>GSSMASGISVEELLKLAKAAYYSGTTVEEAYKLALKLGISVEELLKLAEAAYYSGTTVEEAYKLALKLGISVEELLKLAKAAYYSGTTVEEAYKLALKLGISVEELLKLAKAAYYSGTTVEEAYKLALKLGISVEELLKLAEAAYYSGTTVEEAYKLALKLGISVEELLKLAKAAYYSGTTVEEAYKLALKLGISVEELLKLAKAAYYSGTTVEEAYKLALKLGISVEELLKLAEAAYYSGTTVEEAYKLALKLGISVEELLKLAKAAYYSGTTVEEAYKLALKLGISVEELLKLA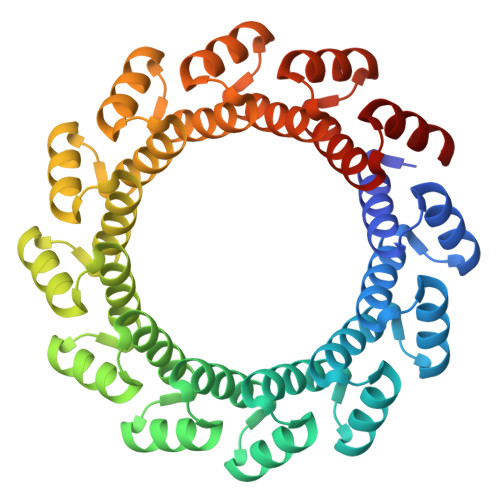KAAYYSGTTVEEAYKLALKLGISVEELLKLAEAAYYSGTTVEEAYKLALKLGISVEELLKLAKAAYYSGTTVEEAYKLALKLG[2x]4-[(1E)-3-{[(2E,4E,6E,8S)-8-hydroxy-4-methyldeca-2,4,6-trienoyl]amino}-3-oxoprop-1-en-1-yl]azete-1(2H)-carboxylic 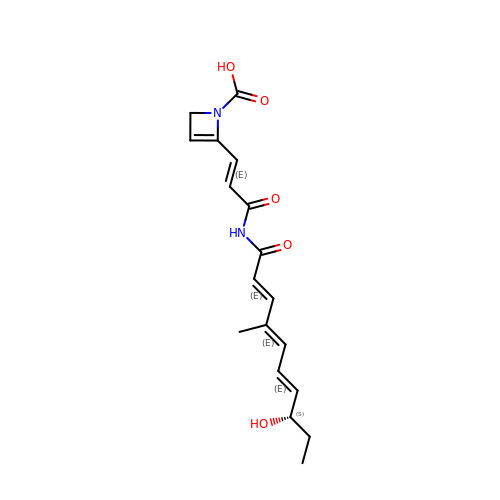acid | C18 H22 N2 O5 | SEMHODIMVPKJPJ-ATTYUXRXSA-N>[8x]MAPTWFYNTTNSEKLRELQHVLGGSAKLGYLTAKVTEILDVDLETVIRAKAIAAYRAVRVPVIVEHGALCIDALNGLPGALVKPFWESLDTRLCEVIPAGQRTARARGALCYCDGRERHVLIEETEGEIAPSARGTGGFHWDPIFIPKGQTRTFAEMSLDEKLSFSPLGRLHTRLRTELGL;>MTTLTLSEAAPLLKKEFREGRLIPFLGAGFSKPLKLPDGSQLIASLAKTLGFEPELFDMHG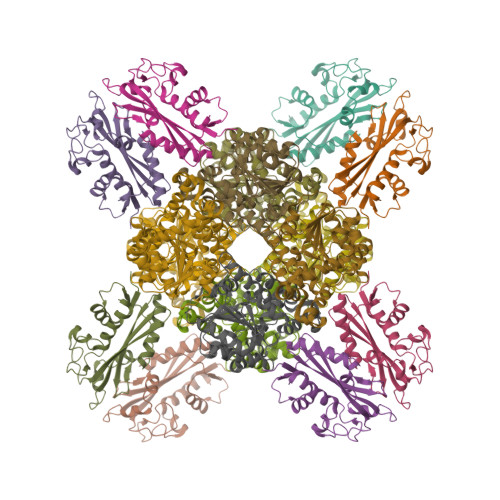RFEQLAEFFAISAPNRLQRLVYEMSLSFDSAEAEALREKSPMHRALAALDWRTIYTTNYDKHVEGALRDAGKQAAVLASFADFQGPRARDVCEVIKFHGTLDQPDTIVLTESSYFQRMALDAPPDQRLRADLLANSFLFIGYSFSDTNIRYIWYRMNQLREQSQLGVKHSQARRCFFATHGAGLVQPDILQQWNIDVIQLDPTDKSASVARLLESIA[8x]>[10x]QTDMSRKAFVFPKESDTSYVSLKAPLTKPLKAFTVCLHF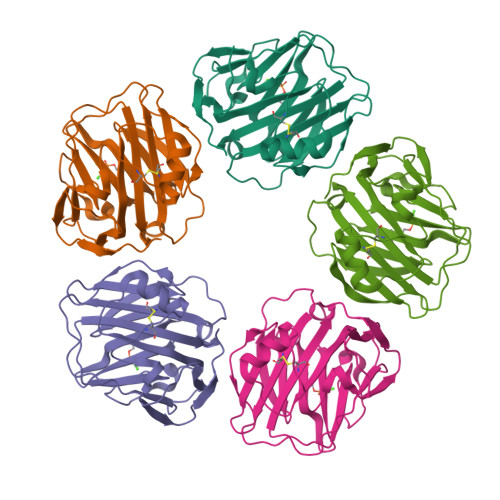YTELSSTRGYSIFSYATKRQDNEILIFWSKDIGYSFTVGGSEILFEVPEVTVAPVHICTSWESASGIVEFWVDGKPRVRKSLKKGYTVGAEASIILGQEQDSFGGNFEGSQSLVGDIGNVNMWDFVLSPDEINTIYLGGPFSPNVLNWRALKYEVQGEVFTKPQLWP ABC transporters form one of the largest transporter gene families and use ATP to power the movement of a wide range of substrates across the membranes of both prokaryotic and eukaryotic cells. The TMDs bind the transported substrate and the NBDs provide the energy necessary for transport by binding and hydrolyzing two (or sometimes just one) molecules of ATP. We have solved the structure of the native nucleotide-binding domain, FbpC, from the N. gonorrhoeae iron-uptake ABC transporter, FbpABC (Lau et al., 2004). The first 240 amino acids of each FbpC monomer show the same overall ATPase topology and sequence motifs previously observed for other NBD structures from ABC transporters (Oswald et al., 2006).

FbpC consists of 352 amino acids and the structure shows a domain-swapped physiological dimer in the asymmetric unit cell (Smith et al., 2002). The crystal structure was determined to a final resolution of 1.9 Å and refined to a working R factor of 18.6% and Rfree of 23.4%. A notable feature of the FbpC structure is that it is trapped in the ATP-bound prehydrolysis state with a divalent metal ion cofactor, even though the protein is an active ATPase (Lau et al., 2004). A divalent metal ion is found coordinated between the β- and γ-phosphates of each ATP and the Q-loop glutamine (Gln87) in the electron density maps of FbpC. Given the high concentration of calcium in the crystallization conditions (0.2 M), it is highly probable that the ions observed in the active site of this structure are calcium. A striking feature of the FbpC active site is that neither of these residues makes any interaction with each other or the γ-phosphate of ATP. This suggests that the presence of calcium in the cofactor-binding site may have caused the catalytic dyad of His197 and Glu164 to adopt an unproductive conformation, although His197 still makes the trans interactions to the carbonyl oxygens of Ser167 and Leu169 on the D-loop of the opposing monomer as observed in HlyB. FbpC also contains an additional C-terminal regulatory domain of ∼110 amino acids (RD; residues 242–352) that adopts two OB-folds per monomer. Unlike MalK, the domains in FbpC undergo a substantial domain swap between the two monomers.

>MTAALHIGHLSKSFQNTPVLNDISLSLDPGEILFIIGASGCGKTTLLRCLAGFEQPDSGEISLSGKTIFSKNTNLPVRERRLGYLVQEGVLFPHLTVYRNIAYGLGNGKGRTAQERQRIEAMLELTGISELAGRYPHELSGGQQQRAALARALAPDPELILLDEPFSALDEQLRRQIREDMIAALRANGKSAVFVSHDREEALQYADRIAVMKQGRILQTASPHELYRQPADLDAALFIGEGIVFPAALNADGTADCRLGRLPVQSGAPAGTRGTLLIRPEQYSLHPHSAPAASIHAVVLKTTPKARHTEISLRAGQTVLTLNLPSAPTLSDGISAVLHLDGPALFFPGNTLEHHHHHH[2x]propyl 4-(4-chloranyl-2-phenyl-quinolin-7-yl)carbonylpiperazine-1-carboxylate 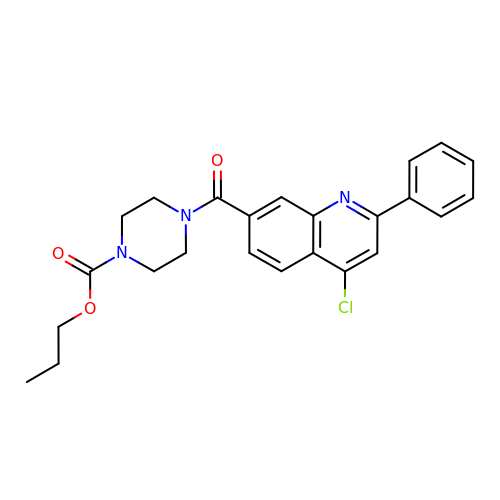| C24 H24 Cl N3 O3 | KSURKAFQFJOCBC-UHFFFAOYSA-N> MSVIHPLQNLLTSRDGSLVFAIIKNCILSFKYQSPNHWEFAGKWSDDFDKIQESRNTTAKEQQGQSSENENENKKLKSNKGDSIKRTAAKVPSPGLGAPPIYSYIRNLRLTSDESRLIACADSDKSLLVFDVDKTSKNVLKLRKRFCFSKRPNAISIAEDDTTVIIADKFGDVYSIDINSIPEEKFTQEPILGHVSMLTDVHLIKDSDGHQFIITSDRDEHIKISHYPQCFIVDKWLFGHKHFVSSICCGKDYLLLSAGGDDKIFAWDWKTGKNLSTFDYNSLIKPYLNDQHLAPPRFQNENNDIIEFAVSKIIKSKNLPFVAFFVEATKCIIILEMSEKQKGDLALKQIITFPYNVISLSAHNDEFQVT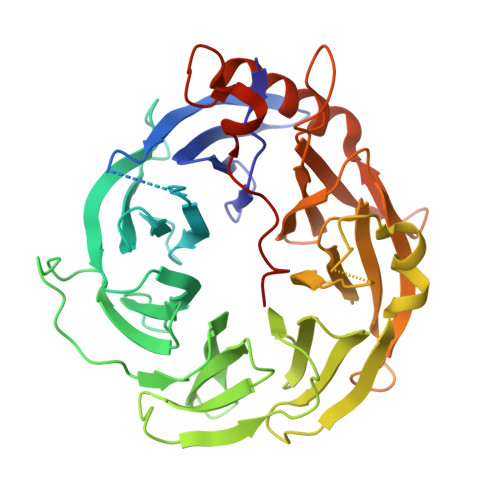LDNKESSGVQKNFAKFIEYNLNENSFVVNNEKSNEFDSAIIQSVQGDSNLVTKKEEIYPLYNVSSLRKHGEHYSHHHHHH>[6x]SMFEIKKICCIGAGYVGGPTCSVIAHMCPEIRVTVVDVNESRINAWNSPTLPIYEPGLKEVVESCRGKNLFFSTNIDDAIKEADLVFISVNTPTKTYGMGKGRAADLKYIEACARRIVQNSNGYKIVTEKSTVPVRAAESIRRIFDANTKPNLNLQVLSNPQFLAEGTAIKDLKNPDRVLIGGDETPEGQRAVQALCAVYEHWVPREKILTTNTWSSEL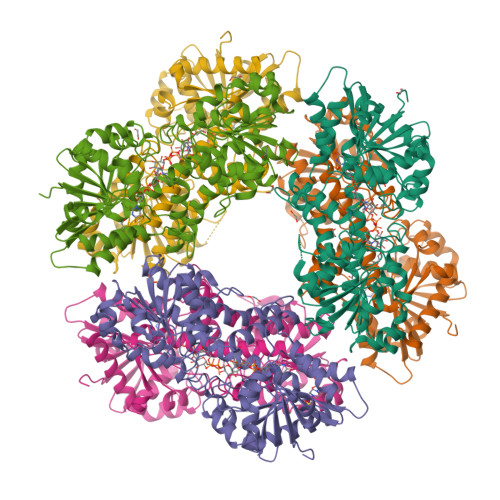SKLAANAFLAQRISSINSISALCEATGADVEEVATAIGMDQRIGNKFLKASVGFGGSCFQKDVLNLVYLCEALNLPEVARYWQQVIDMNDYQRRRFASRIIDSLFNTVTDKKIAILGFAFKKDTGDTRESSSIYISKYLMDEGAHLHIYDPKVPREQIVVDLSHPGVSEDDQVSRLVTISKDPYEACDGAHAVVICTEWDMFKELDYERIHKKMLKPAFIFDGRRVLDGLHNELQTIGFQIETIGKKV>[2x]MRLDLDFG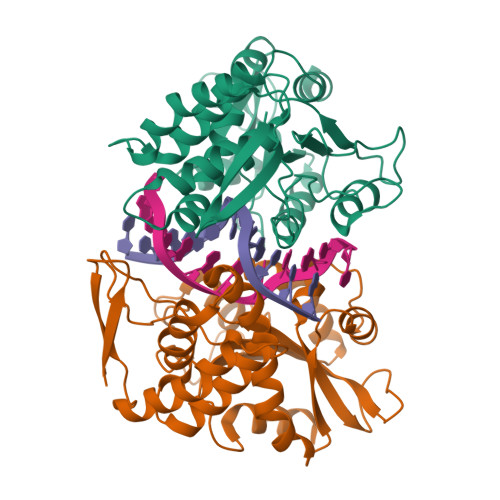RGLVAHVMLDNVSEEQYQQISDYFVPLVNKPKLKSRDAIGQAFVMATEVCPDANPSDLWHHVLYRIYIREKIGTDPSQSWVRTSGEAFEVALVERYNPVLARHGIRLTALFKGQKGLALTRMGVADRVGSRKVDVMIEKQGGGRSPDAEGFGVVGGIHAKVSLAERVSDDIPASRIMMGEGLLSVLSTLDVKSFPPPHGDLVNRGELGTPDRPSDKRNYIEGHGDFSACFSYNLRTSPSNATTPSGRHIYVSGFSGQDDEFTDYLVAQLA> ATETSFIIDA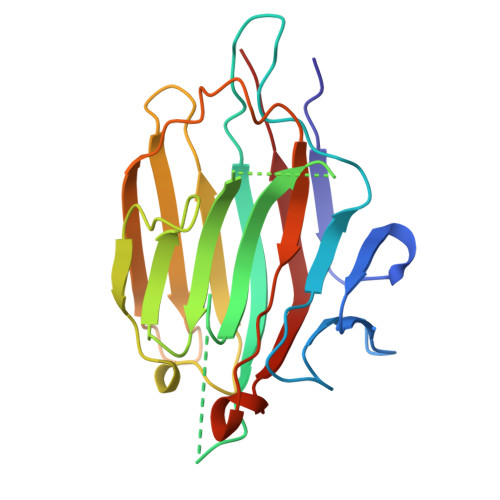FNKTNLILQGDATVSSNGNLQLSYNSYDSMSRAFYSAPIQIRDSTTGNVASFDTNFTMNIRTHRQANSAVGLDFVLVPVQPESKGDTVTVEFDTFLSRISIDVNNNDIKSVPWDVHDYDGQNAEVRITYNSSTKVFSVSLSNPSTGKSNNVSTTVELEKEVYDWVSVGFSATSGAYQWSYETHDVLSWSFSSKFI>[3x]GAMTSSVNELENWSKWMQPIPDSI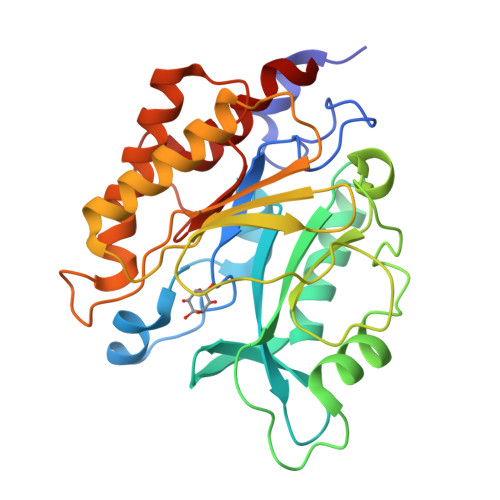PLARISIPGTHDSGTFKLQNPIKQVWGMTQEYDFRYQMDHGARIFDIRGRLTDDNTIVLHAGPLYLYVTLHEFINEAKQFLKDNPSETIIMSLKKEYEDMKGAEDSFSSTFEKKYFVDPIFLKTEGNIKLGDARGKIVLLKRYSGSNEPGGYNNFYWPDNETFTTTVNQNANVTVQDKYKVSYDEKVKSIKDTMDETMNNSEDLNHLYINFTSLSSGGTAWNSPYYYASYINPEIANYIKQKNPARVGWVIQDYINEKWSPLLYQEVIRANKSLIKE> MWSHPQFEKSTPLRDEVTDKNYYYLFDKKSFFNGKALNNAIPGGPKFEPLYPREEEEDYNEFNSIDRVIFRVPIRSEYKVAFPHLYNSRPRSVRIPWYNNPVSCIIQNDEEYDTPALFFDPSLNPIPHFIDNNSSLNVSNTKENGDFTLPEDFAPLLAEEEELILPNTKDAMSLYHSPFPFNRTKGKMVRAQDVALAKKWFLQHPDEEYPVKVKVSYQKLLKNYVLNELHPTLP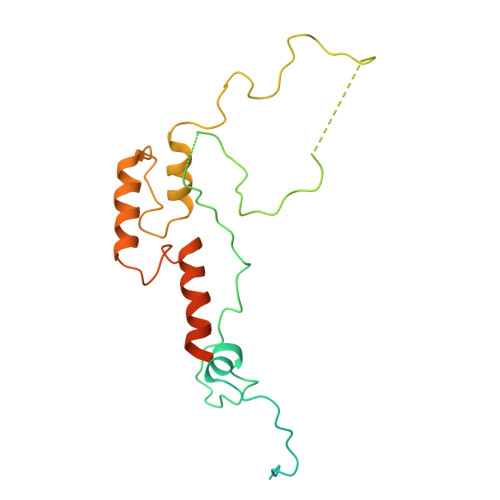TNHNKTKLLKSLKNTK Here we report the cryo-EM structure and biochemistry characterization of gp105, a protein that is encoded by the jumbo phage 201φ2-1 and is involved in the formation of the nucleus-like compartment in phage 201φ2-1 infected Pseudomonas chlororaphis. The nucleus-like compartments are assembled mainly by a phage-encoded nucleus-like shell protein (NLSP). Previous studies using mass spectrometry analysis identified the phage-encoded gene product 105 (gp105) as the major component of the nucleus-like shell. Gp105 has 631 amino acids and shares sequence homology with other NLS proteins (Chaikeeratisak et al., 2017a,b).

The four molecules at the interface of two head-to-tail tetramers sit on a 2-fold axis, interact with each other through one distal end of the molecule and form a concave tetramer. Given that some of the concave tetramers can have a stable conformation, we performed locally focused classifications and refinements on the concave tetramers with C2 symmetry imposed. Through several rounds of classifications and refinements, we finally obtained a reconstruction of the concave tetramer at a resolution of 4.09 Å. The structure of gp105 is composed of N- and C- two domains. The N-terminal domain (NTD) contains a β sheet core of 4 antiparallel β strands that is sandwiched by 3 α helices. The C-terminal domain (CTD) contains a twisted β sheet core of 7 antiparallel β strands that is sandwiched by 10 α helices. Interactions between molecule A and the two neighboring molecules B and B’ are mediated mainly by loop 303–320 (molecule A), loop 273–287 (molecule B’), the N-terminal segment (residues 49–61, molecule A), and the C-terminal fragment (residues 589–610, molecule B). The C-terminal segment (CTS: residues 589–610) of molecule B is inserted into a groove of the CTD from molecule A. Hydrophobic residues, including F592, M593, V597, V603, A607, and V609, are involved in the interactions between molecule A and the CTS of molecule B. The interaction mediated by the CTS, the loop 303–320, and loop 137–155 are unique and only exist in between the molecules of the concave tetramers. In the high-resolution concave tetramer structure we obtained, the angle between the planes calculated with the subunits AB’ and A’B, respectively, is approximately 85.5 degrees, and the distance between the gravity centers of the subunits AB’ and A’B is approximately 58.9 Å. Thus, the concave tetramers play a key role in regulating the size and curvature of the gp105 assemblies.

>[4x]MIRDTATNTTQTQAAPQQAPAQQFTQAPQEKPMQSTQSQPTPSYAGTGGINSQFTRSGNVQGGDARASEALTVFTRLKEQAVAQQDLADDFSILRFDRDQHQVGWSSLVIAKQISLNGQPVIAVRPLILPNNSIELPKRKTNIVNGMQTDVIESDIDVGTVFSAQYFNRLSTYVQNTLGKPGAKVVLAGPFPIPADLVLKDSELQLRNLLIKSVNACDDILALHSGERPFTIAGLKGQQGETLAAKVDIRTQPLHDTVGNPIRADIVVTTQRVRRNGQQENEFYETDVKLNQVAMFTNLERTPQAQAQTLFPNQQQVATPAPWVASVVITDVRNADGIQANTPEMYWFALSNAFRSTHGHAWARPFLPMTGVAKDMKDIGALGWMSALRNRIDTKAANFDDAQFGQLMLSQVQPNPVFQIDLNRMGETAQMDSLQLDAAGGPNAQKAAATIIRQINNLGGGGFERFFDHTTQPILERTGQVIDLGNWFDGDEKRDRRDLDNLAALNAAEGNENEFWGFYGAQLNPNLHPDLRNRQSRNYDRQYLGSTVTYTGKAERCTYNAKFIEALDRYLAEAGLQITMDNTSVLNSGQRFMGNSVIGNNMVSGQAQVHSAYAGTQGFNTQYQTGPSSFYALEHHHHHH>MALTATVRRAEL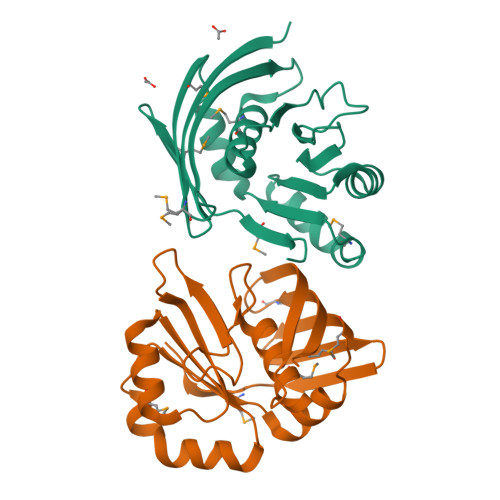QISDMDRGYYANHSLTLAQHPSETDERLMVRLLAFALFADDRLEFGRGLSNDDEPDLWRRDYTGDPDLWIDLGQPDESRVRKACNRSREAVVIGYGGQATETWWKKHANAMGRYRNLRVIELDSQATEALGALIQRGMRFDVIIQDGEVQMLADHGSVTLTPMVRQAPAE[2x]> EDPQQV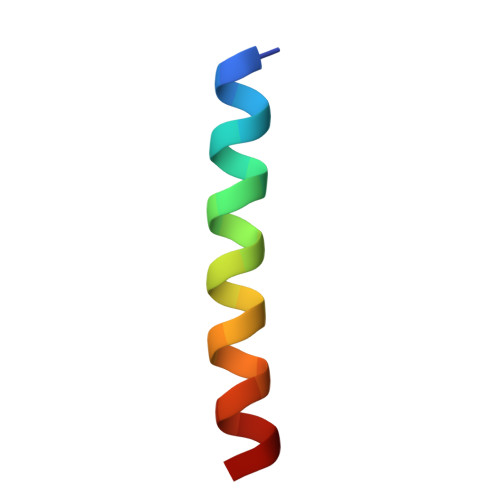FDERIKFANQLHDEYLVS> NAQPNLGRSTKA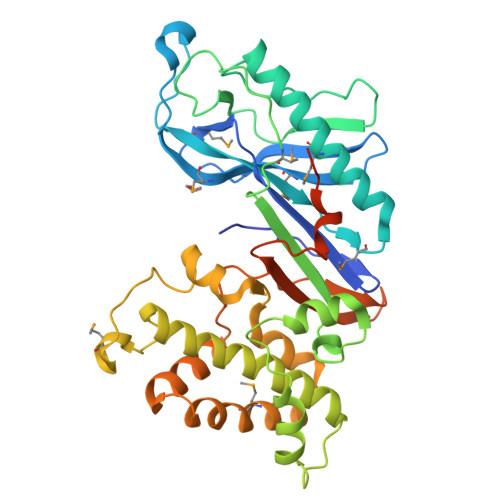TPDFPTHFPKSSIGIENELAGLVVAMPANSAQKFGYVKSAQGDALFMLTKDMNQGSYQRPPSLQDGKNYQNWQTHTVELVSYPCEMDDKAAVETRKQAMLWLATHFTTHIDQSNHQPLAPIQSEDGRFVIEITNAKHVIAAGNGISAESQGQTITMTPSGQQATVGVAAKGFGTSATPELRLLESAPWYQKSLKSQFASLTSAENLDDKELAANVFAYLTSIYLKTAELAKKFGIYINEWDPMSEQITPNANGLTDPKVKNAWEILPRTKPSKIVEILSKSDAKAVMKHIKPQLQSRYSESLSKNVFQYFQDGGEVAGHGINNATVGDKHSPELAILFEFRTVPNELQSYLPKTESTTKSEVKLLDQFDPMKRKTVIQQVESLV> GPGSEFGPRRPFQQKPLQLWSKFDVGDWLESIHLGEHRDRFED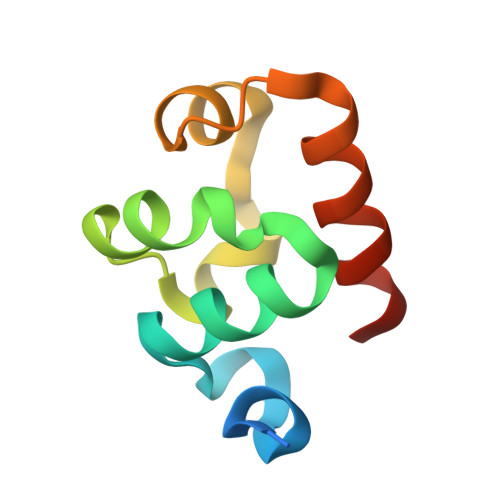HEIEGAHLPALTKEDFVELGVTRVGHRMNIERALRQLDGS>[4x]MRKLNPALEFRDFIQVLKDEDDLIEITEEIDPNLEVGAIMRKAYESHLPAPLFKNLKGASKDLFSILGCPAGLRSKEKGDHGRIAHHLGLDPKTTIKEIIDYLLECKEKEPLPPITVPVSSAPCKTHILSEEKIHLQSLPTPYLHVSDGGKYLQTYGMWILQTPDKKWTNWSIAAGMVVDDKHITGLVIKPQHIRQIADSWAAIGKANEIPFALCFGVPPAAILVSSMPIPEGVSESDYVGAILGESVPVVKCETNDLMVPATSEMVFEGTLSLTDTHLEGPFGEMHGYVFKSQGHPCPLYTVKAMSYRDNAILPVSNPGLCTDETHTLIGSLVATEAKELAIESGLPILDAFMPYEAQALWLILKVDLKGLQALKTTPEEFCKKVGDIYFRTKVGFIVHEIILVADDIDIFNFKEVIWAYVTRHTPVADQMAFDDVTSFPLAPFVSQSSRSKTMKGGKCVTNCIFRQQYERSFDYITCNFEKGYPKGLVDKVNENWKRYGYKHHHHHH

The UbiD superfamily is composed of a wide variety of (de)carboxylases acting on aromatic, hetero-aromatic, and unsaturated aliphatic acids. Prenylated FMN consists of an FMN molecule modified by the addition of a fourth non-aromatic ring joined via N5–C1′ and C6–C3′ linkages between the flavin and prenyl moieties. Following binding of prFMNreduced and formation of holo-UbiD, the cofactor undergoes oxidation to form the catalytically relevant oxidized prFMN species. In the UbiD enzyme family, Arg173, Glu277, and Glu282 (A. niger Fdc1 numbering) form a conserved ionic network.

The corresponding six variants were also made in the related S. cerevisiae Fdc1, with the corresponding UV-visible spectra, decarboxylation assays (of cinnamic acid), and crystal structures revealing trends similar to those observed for the A. niger variants. As observed for A. niger Fdc1, the R175A mutant (S. cerevisiae numbering) shows a prominent 550-nm peak, indicating the presence of prFMNradical; however, this feature is absent in the R175K variant. Activity cannot be detected for R175A, which is consistent with the presence of prFMNradical indicated by the UV-visible spectrum. Crystallization of wildtype, E285D, and R175A S. cerevisiae Fdc1 variants confirms cofactor incorporation. The crystal structure of the R175A variant again shows prFMN in an unmodified form; here disruption of the ERE hydrogen bonding network has resulted in residue Glu285 moving away from the active site to within hydrogen-bonding distance (2.7 Å) of residue His287.~{N}-(1,4-dimethyl-2-oxidanylidene-quinolin-7-yl)ethanamide | C13 H14 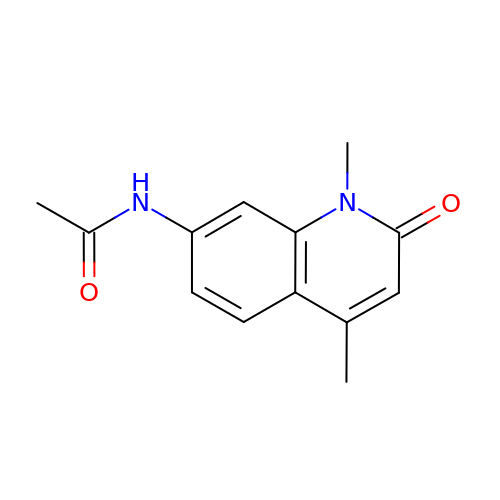N2 O2 | YAOZNWQIDDSLHQ-UHFFFAOYSA-N3-amino-5-[(4-chlorophenyl)amino]-N-(propan-2-yl)-1H-1,2,4-triazole-1-carboxamide | C12 H15 Cl N6 O | 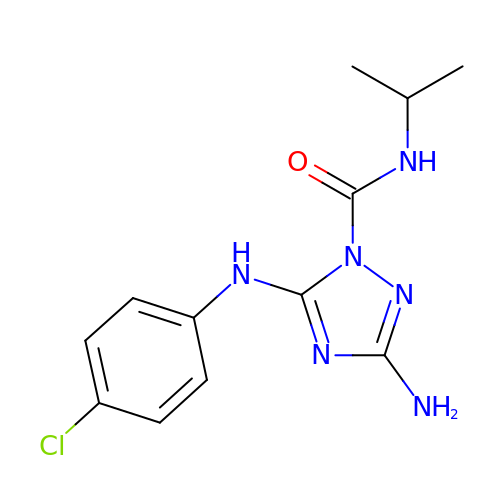WQFRHSPASBOZIT-UHFFFAOYSA-N Many invasive bacteria block the initial mucosal host response during colonization by cleaving host immunoglobulin A1 (IgA1) via a bacterially encoded IgA1 protease (IgA1P). Here, we used cryo-EM to characterize the metallo-IgA1P of a more distantly related family member from Gemella haemolysans, an emerging opportunistic pathogen implicated in meningitis, endocarditis, and more recently bacteremia in the elderly. Third, all M26 metallo-IgA1Ps comprise the M26 region itself that is responsible for IgA1 cleavage, which corresponds to G. haemolysans IgA1P residues 907-2201. The two histidine residues of the HEXXH motif together with a conserved downstream glutamic acid coordinate a Zn ion to polarize the carbonyl group of the substrate’s scissile peptide.

We solved the structure of the G. haemolysans IgA1P catalytic region, G. haemolysans IgA1P residues 907-2201, through cryo-EM single particle reconstruction. A cryo-EM 3D reconstruction of this metallo-IgA1P resulted in a 3.2 Å resolution map that readily afforded a near-atomic-resolution model that includes the active site. In regard to similarities that exclude the NTD2 gating domain described further below, the G. haemolysans IgA1P NTD1, MD, and CTD superimpose well with their analogous domains within the S. pneumoniae IgA1P with an RMSD of 1.1 Å over all Cα. The RMSD increases to 2.3 Å over all Cα atoms when including the NTD2, which is further discussed below in regard to differences. Specifically, residues comprising the conserved metalloprotease signature HEMTH motif (residues 1847-1851) and the downstream E1871 are structurally perfectly aligned with those within S. pneumoniae IgA1P. The most striking difference between the two substrate-free IgA1Ps is that the G. haemolysans IgA1P NTD2 gating domain is shifted to a more open position by ~6 Å relative to that of S. pneumoniae IgA1P. The large shift of the G. haemolysans IgA1P NTD2 can be viewed as a partially open conformation existing along the conformational continuum between the substrate-free and substrate-bound states. Interestingly, both metallo-IgA1Ps comprise an extended structure within their active site that are residues 1296-1308 in G. haemolysans IgA1P (corresponding to residues 1054-1063 in S. pneumoniae IgA1P), which would occlude substrate entry. For example, the gating mechanism could subscribe to an inherent opening/closing (opening/closing of the “gate”). However, this partial opening does not give any measurable advantage in binding affinity described above for the G. haemolysans IgA1P inactive mutant over that of its S. pneumoniae IgA1P counterpart. Specifically, our findings reveal that despite the substrate-free G. haemolysans IgA1P structure showing a more open active site relative to that of the S. pneumoniae IgA1P, substrate binding is still necessary to further open the active site to facilitate access to the hinge region of the shared IgA1 substrate.

> MRKYLEEKYNKFSLRKLTVGVCSMTIGSFFLVSTVQPEDYVVKAADNAIVHYKYVGEDNLTDKEKELIKKEVPSVVSSKEETYYLVFKPTKTTQLNKLPNTGLNYGVGSMLLGGMLGLVVVVVAKGKNKSRKILSILLVTSLGATTLELPARAMEDLQLSVYNMDYNLKVGDKLPEISSIPGYSFVGFIKNEAETKKENEEVKEQITSQQHNKKQPELKENTDENVIENKQENKTTLKISDKKEDKKVIENINKKDEKKVQGVNTVNPQDEVLAGKLTKPELLYSDKIIETPLKYNQIIESNDQLPEGTTRIKQQGKEGKKTEVIRMFTVEGKEVSRELISTKTEEPVSEIIEKGTKKAVSNVITKGQKLVKPAVEVKPEYTGVQAGAIVEPVKAEVPKEYTGVQAGAIVEPAKVETPKEYTGVQAGAIVEPAKAEVSKEYTGVQAGTIVEPAKAEVPKEYTGVQAGAIVEPEKVEPQYGGVTSGALVKPEKIEAPKEYTGVQAGAVVEPAKAEAPKEYRGVQAGAIVEPEKIESPKEYTGVQAGAVVEPAKAEVPKEYRGVQAGAIVEPEKIESPKEYTGEQSGAIVEPEKVETTKEYTGIQAGALVEPEKVEAPKEYTGVQAGAIVEPEKVEPPKEYTGVQAGAIVEPEKVEAPKEYTGKIEPLKTENPKPTVENNNTAEINNVPKNASALLRMNFVKGNQVLSGTGSATFIAPNVLLTVAHNFINNSADNSTGEFIGDKSKNTYEWQTPDGQKGSFTSEDIHFYNKKDYPKGFIYDLAVITLPQSTRRQHANLVENYSKVNVNDKLNVYGYPRGEYAHLKDTTVEIEQKYANNTYGVQYQGGKAGMSGGGIFNSKGEVIGLHQNGAENRSGGLILSPTQLDWIRSIIKGKEITPNYDALERHKDEKKDDIKEEKQVDKKLELRNISNVELYTLENNKYRHVSSLSSVPTNPEAYFMKVKSENFKDVMLPVKSIESARKDNQDVYKIVGQANDLIQHENNITLENYTYYLPKTVNSENGVYTSFKNLVDAMNINPYGTFRLGATMDAREVELSDGQESYINKEFSGKLIGENKGKYYAIYNLKKPLFKALSHATIQDLSIKEANVSSKEDAATIAKEAKNDTTIANVHSSGVIAGERSIGGLISQVTDSTISNSSFTGRITNTYDTTATYQIGGLVGKLSGVGALIEKSISSIDMATNANTGDQVVGGVAGVVDKKATIRNSYVEGNLNNVKPFGKVGGVVGNLWDRETSEVSNSGNLTNVLSDVNVTNGNAIAGYDFNGIKATNTYSNKNNKVVKVVQVDDEVLSKDSEEQRGTVLENNIVLEKKIELVPKKNTKIEDFNFSSRYETDYKNLKDADVSRLRVYKNIEKLLPFYNRETIVKYGNLVDANNTLYTKDLVSVVPMKDKEVISDINKNKTSINKLLLHYSDNTSQTLDIKYLQDFSKVAEYEIANTKLIYTPNTLLHSYNNIVKAVLNDLKSVQYDSDAVRKVLDISSNIKLTELYLDEQFTKTKANIEDSLSKLLSADAVIAENSNSIIDNYVIEKIKNNKEALLLGLTYLERWYNFKYDNTSAKDLVLYHLDFFGKSNSSALDNVIELGKSGFNNLLAKNNVITYNVLLSKNYGTEGLFKALEGYRKVFLPNVSNNDWFKTQSKAYIVEEKSTIPEVSSKQSKQGTEHSIGVYDRLTSPSWKYQSMVLPLLTLPEEKMIFMIANISTIGFGAYDRYRSSEYPKGDKLNRFVEENAQAAAKRFRDHYDYWYKILDKENKEKLFRSVLVYDAFRFGNDTNKETQEANFETNNPVIKNFFGPAGNNVVHNKHGAYATGDAFYYMAYRMLDKSGAVTYTHEMTHNSDREIYLGGYGRRSGLGPEFYAKGLLQAPDHSYDPTITINSVLKYDDSENSTRLQIADPTQRFTNVEDLHNYMHNMFDLIYTLEILEGRAVAKLDYNEKNDLLRKIENIYKKDPDGNSVYATNAVRRLTSDEIKNLTSFDKLIENDVITRRGYIDQGEYERNGYHTINLFSPIYSALSSKIGTPGDLMGRRMAFELLAAKGYKEGMVPYISNQYEKEAKDRGSKIRSYGKEIGLVTDDLVLEKVFNKKYGSWVEFKKDMYKERVEQFSKLNRVSFFDPNGPWGRQKNVTVNNISVLEKMIETAVREDAEDFTAQVYPDTNSRVLKLKKAIFKAYLDQTKDFRTSIFGGK> MISLNGYGRFGLQYVEDRGVGLEDTIISSRLRINIVGTTETDQGVTFGAKLRMQWDDGDAFAGTAGNAAQFWTSYNGVTVSVGNVDTAFDSVALTYASAMGYEASSFGDAQSSFFAYNSKYDASGALDNYNGIAVTYSISGVNLYLSYVDPDQTVDSSLVTEEFGIAADWSNDMISLAAAYTTDAGGIVDNDIAFVGAAYKFNDAGTVGLNWYDNGLSTAGDQVTLYGN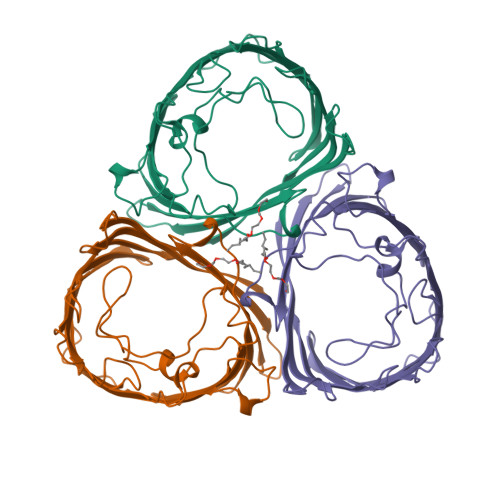YAFGATTVRAYVSDIDRAGADTAYGIGADYQFAEGVKVSGSVQSGFANETVADVGVRFDF>[2x]MNTFDKHDLSGFVGKHLVYTYDNGWNYEIYVKNDNTIDYRIHSGLVGNRWVKDQEAYIVRVGESIYKISWTEPTGTDVSLIVNLGDSLFHGTIFFPRWVMNNPEPTVCFQNDHIPLMNSYREAGPAYPTEVIDEFATITFVRDCGANNESVIACAASELPKNFPDNLK

Ferulic acid decarboxylase (FADase) catalyzes the non-oxidative decarboxylation of ferulic acid to produce 4-vinylguaiacol. To understand the detailed mechanism of action of FADase from Enterobacter sp. Px6-4, we cloned and expressed the FADase gene in E. coli BL21 (DE3) and solved the crystal structures of FADase and FADase in complex with a substrate analog sodium ferulate. The cylinder-shaped monomer of FADase had an overall dimension of 25×25×45 Å and is composed of nine β-strands, two α-helices and two η-helices. The FADase molecule could be divided into three independent components: the core, a helical bottom, and a C terminal extension.

The crystal structures were determined to 2.4 Å and 2.1 Å resolutions respectively for the pure FADase and FADase complexed with sodium ferulate. There were two molecules in one asymmetric unit with a Matthews coefficient of 2.6 at 46% solvent content. The result was consistent with the dimerization state of FADase, which was first observed in gel-filtration chromatography and supported further by crosslinking with ethylene glycolbis. The results also suggested that the biologically active form for FADase was a homodimer. The core was formed by anti-parallel β1 to β9, which together form an open-ended β-barrel. The helical bottom, composed of α1, α2 and η1, η2, was located at the bottom of the core β-barrel. The catalytic center was located between the core β-barrel and the helical bottom and was surrounded by α2, β8, β9, and the hair-pins between β1/2 and β3/4. The C terminal extension, which contained a long coil with η2 in the middle, was located behind β9. Comparison of the crystal structures of pure FADase and FADase in complex with sodium ferulate revealed that an active hydrophobic pocket was formed when FADase crystals were soaked in a solution containing sodium ferulate. In the closed form, the two hair-pins moved towards β9 by about 5 Å to seal the pocket and shield the substrate away from the catalytic center.2'-O-[(5'-PHOSPHO)RIBOSYL]ADENOSINE-5'-MONOPHOSPHATE 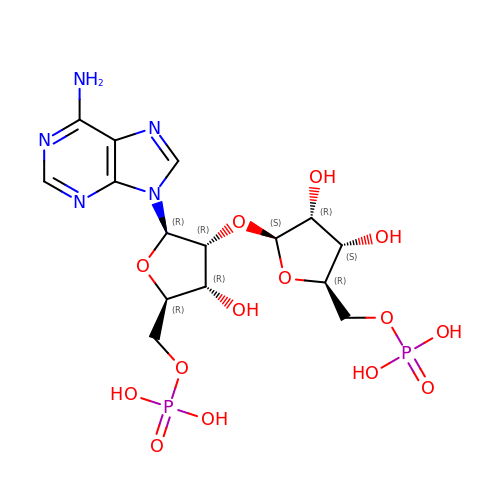| C15 H23 N5 O14 P2 | BHIWBSNWEZIHHL-ZQSHOCFMSA-N> IIGGTECKPHSRPYMAYLEIVTSNGPSKFCGGFLIRRNFVLTAAHCAGRSITVTLGAHNITEEEDTWQKLEVIKQFRHPKYNTSTLHHDIMLLKLKEKASLTLAVGTLPFPSQFNFVPPGRMCRVAGWGRTGVLKPGSDTLQEVKLRLMDPQACSHFRDFDHNLQLCVGNPRKTKSAFKGDSGGPLLCAGAAQGIVSYGRSDAKPPAVFTRISH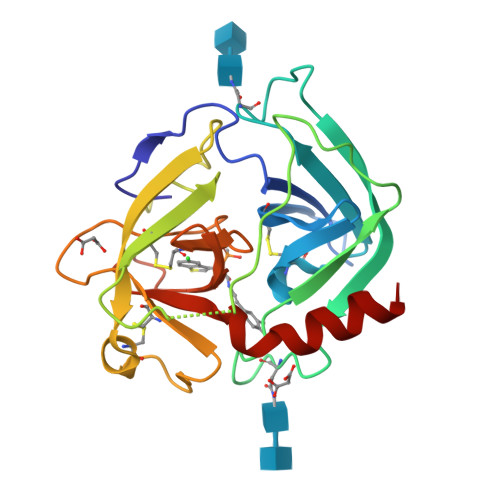YQPWINQILQAN> DPSKDSKAQVSAAEAGITGTWYNQLGSTFIVTAGADGALTGTYESAVGNAESRYVLTGRYDSAPATDGSGTALGWTVAWKNNYRNAHSATTWSGQ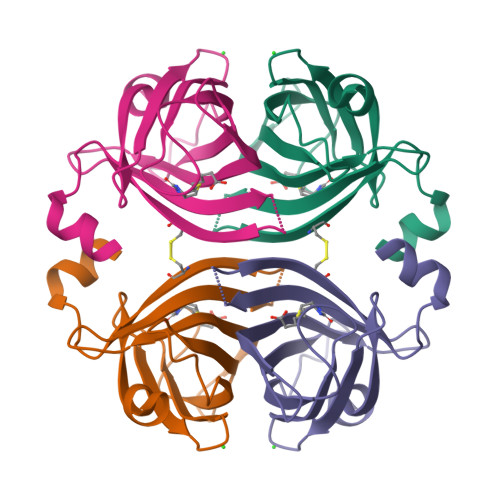YVGGAEARINTQWLLTSGDSSNGSDGSTLVGCDTFTKVKPSAASIDAAKKAGVNNGNPLDAVQQ(2S)-{[(2S,3S,4S)-2-amino-4-hydroxy-4-(5-hydroxypyridin-2-yl)-3-methylbutanoyl]amino}[(2R,3S,4R,5R)-5-(2,4-dioxo-3,4-dihydropyrimidin-1(2H)-yl)-3,4-dihydroxyoxolan-2-yl]acetic 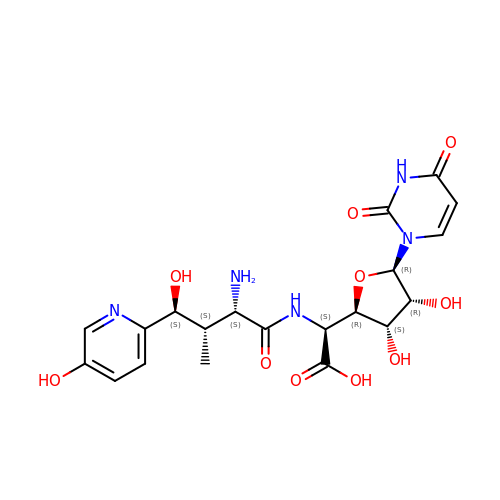acid (non-preferred name) | C20 H25 N5 O10 | WWJFFVUVFNBJTN-VHDFTHOZSA-N> MANLKEIRAKVASIKSTQKITRAMQMVAASKMRRAQERMAQGRPYADNMRRVIAHLVQANPEYKHRYMVDRPVKRVGYIIVSSDRGLAGGLNINLFKKVVQHVKAQQEQSIEVQFALIGQKAVSFFKNYGGKVLGATTQIGDAPSLEQLTGSVQVMLDAFDKGELDRIYLVSNGFVNAMTQKPKVEQLVPLAPAEEGDDLN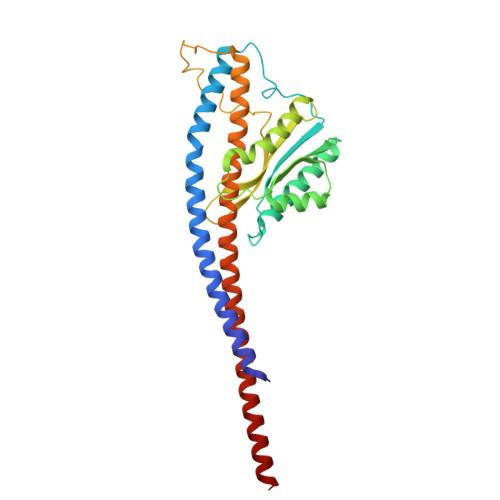RTYGWDYIYEPEAEELLNGLLVRYIESMVYQGVIENVACEQSARMVAMKAATDNAGQLIKDLQLIYNKLRQAAITQEISEIVGGAAAV>XSSQVEHPAGGYKKLFETVEELSSPLTAHVTGRIPLWLTGSLLRCGPGLFEVGSEPFYHLFDGQALLHKFDFKEGHVTYHRRFIRTDAYVRAMTEKRIVITEFGTCAFPDPCKNIFSRFFSYFRGVEVTDNALVNIYPVGEDYYACTETNFITKVNPETLETIKQVDLCNYVSVNGATAHPHIENDGTVYNIGNCFGKNFSIAYNIVKIPPLQADKEDPISKSEIVVQFPCSDRFKPSYVHSFGLTPNYIVFVETPVKINLFKFLSSWSLWGANYMDCFESNETMGVWLHIADKKRKKYINNKYRTSPFNLFHHINTYEDHEFLI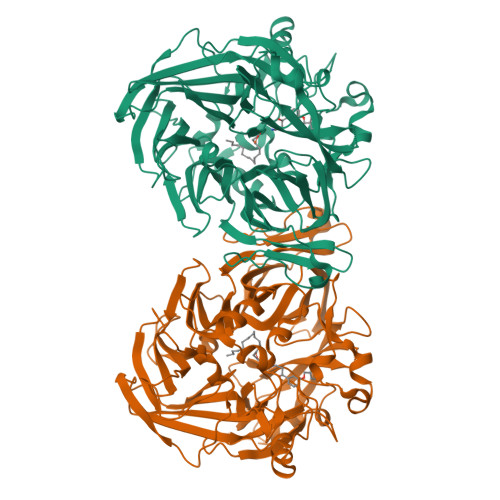VDLCCWKGFEFVYNYLYLANLRENWEEVKKNARKAPQPEVRRYVLPLNIDKADTGKNLVTLPNTTATAILCSDETIWLEPEVLFSGPRQAFEFPQINYQKYGGKPYTYAYGLGLNHFVPDRLCKLNVKTKETWVWQEPDSYPSEPIFVSHPDALEEDDGVVLSVVVSPGAGQKPAYLLILNAKDLSEVARAEVEINIPVTFHGLFKKS[2x]(2~{S})-2-[[(2~{S})-3-azanyl-2-[[oxidanyl(phenylmethoxycarbonylaminomethyl)phosphoryl]amino]propanoyl]amino]-4-methyl-pentanoic 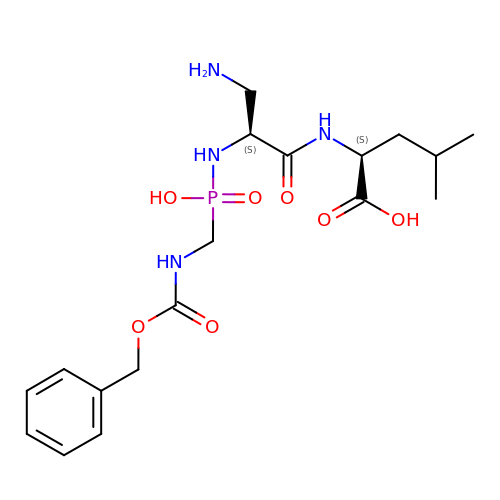acid | C18 H29 N4 O7 P | XZHIMTMEWJSRRL-GJZGRUSLSA-N> MASVHGTTYELLRRQGIDTVFGNPGSNELPFLKDFPEDFRYILALQEACVVGIADGYAQASRKPAFINLHSAAGTGNAMGALSNAWNSHSPLIVTAGQQTRAMIGVEALLTNVDAANLPRPLVKWSYEPASAAEVPHAMSRAIHMASMAPQGPVYLSVPYDDWDKDADPQSHHLFDRHVSSSVRLNDQDLDILVKALNSASNPAIVLGPDVDAANANADCVMLAERLKAPVWVAPSAPRCPFPTRHPCFRGLMPAGIAAISQLLEGHDVVLVIGAPVFRYHQYDPGQYLKPGTRLISVTCDPLEAARAPMGDAIVADIGAMASALANLVEESSRQLPTAAPEPAKVDQDAGRLHPETVFDTLNDMAPENAIYLNESTSTTA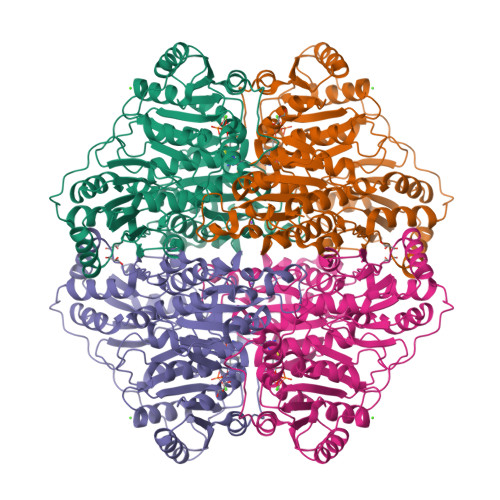QMWQRLNMRNPGSYYFCAAGGTGFALPAAIGVQLAEPERQVIAVIGDGSANYSISALWTAAQYNIPTIFVIMNNGTYGALRWFAGVLEAENVPGLDVPGIDFRALAKGYGVQALKADNLEQLKGSLQEALSAKGPVLIEVSTVSPVKRSHHHHHH>[3x]MGSSYNDWLKSSYSELKKINIIENLIKENNFARAKMLLNNLDLTTLIKYTELSKTITDFCEEAEQADIWRTHLQNFNEEHFSFEEYPPLTVSQLVKGIYFYGQAAECREEEGKPFGDNELEFLKKS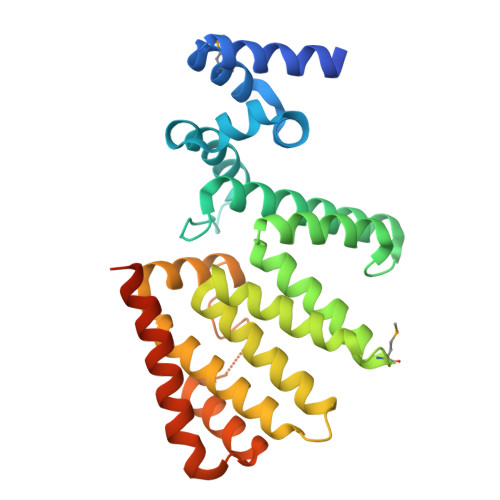AYQHCFYAYNSLSTWAYEKYKMGLNDYSLLTLHYAQKACQYHWTPGYLLFYKTCLNLAILSNAPSLSYQEALEALLIARKLSEHQYSISAINNAYFGKGLIHGNKTQIESWDKAISETIAKGKIPSTLLNKIYDKASEKAKGILDEFTVEVKDMPEEEKLENE>SMTLGYWDIRGLAHAIRLLLEYTDSSYEEKKYTMGDAPDYDRSQWLNEKFKLGLDFPNLPYLIDGAHKITQSNAILCYIARKHNLCGETEEEKIRVDILENQAMDVSNQLARVCYSPDFEKLKPEYLEELPT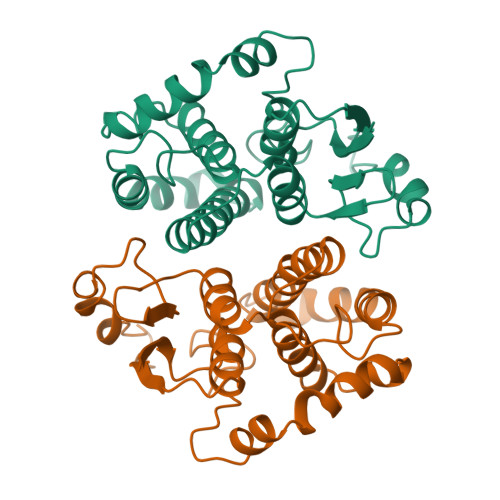MMQHFSQFLGKRPWFVGDKITFVDFLAYDVLDLHRIFEPNCLDAFPNLKDFISRFEGLEKISAYMKSSRFLPKPLYTRVAVWGNK[8x]pmcHuman galectins (GAL) are oligomeric β-galactosidase-binding lectins assembled from small (∼15 kDa) protomeric carbohydrate recognition domains (CRD). Among prototype galectins, galectin-7 (GAL-7) is recognized for its preferential expression profiles in normal epithelial cells. For example, while extracellular GAL-7 can trigger apoptosis of activated T cells following binding to glycoreceptors via its GBS, it can also bind E-cadherin on epithelial cells independently of its GBS. In this work, we studied the impact of homodimer interface mutations on the induction of Jurkat T cell apoptosis, allowing us to positively and negatively modulate the biological activity of GAL-7 by designing a covalent disulfide bridge (G16C) and destabilizing mutation (G16S) to control homodimer strength, stability, and biological activity.

Based on our computational predictions, mutations G16S and F135S should weaken GAL-7 homodimer interactions, while formation of a disulfide bridge in G16C could strengthen protomer interactions and favor GAL-7 homodimer stability. As predicted from our calculations and in support of our MST results, the apo G16C omit map revealed the formation of a Cys16-Cys16 disulfide bridge at the dimer interface. As hypothesized, no binding-associated MST signal was observed for G16C, lending support to stabilization by formation of a disulfide bridge between the two G16C GAL-7 protomers. As expected, the disulfide bridge between the G16C homodimers was found to be a significant contributor to dimer stability. CD melting curves show that G16C is the more stable variant (Tm = 70.0 ± 0.1 °C), followed by WT (Tm = 67.8 ± 0.2 °C) and G16S (Tm = 58.7 ± 0.2 °C). These results confirm the thermal stability advantage conferred by the G16C mutation, which provides a 2.2 °C increase in Tm relative to WT. Conversely, the G16C variant has a greater capacity to induce apoptosis of Jurkat T cells than WT, yielding an EC50 of 5.9 μM (CI95% 5.2–6.7 μM). One of the most significant structural rearrangements between WT and G16X apo structures occurs in the local environment of residues 8–17 (loop 1), which exhibit significant atomic-scale deviations in the variants. This local rearrangement of loop 1 involves Gly16 and its neighboring residues, particularly residues Pro10, Glu11, Gly12, and Arg14.

>[2x]SNVPHKSSLPEGIRPCTVLRIRGLVPPNASRFHVNLLCGEEQGSDAALHFNPRLDTSEVVFNSKEQGSWGREERGPGVPFQRGQPFEVLIIASDDGFKAVVGDAQYHHFRHRLPLARVRLVEVGGDVQLDSVRIF> MPYEIFLAGVVSDNDEAKARAVLGGFTEMREHHRFTRVQHYEPQDIKIRGFPTIKELLKERGPTTALYQELHNILVRQPYTLQI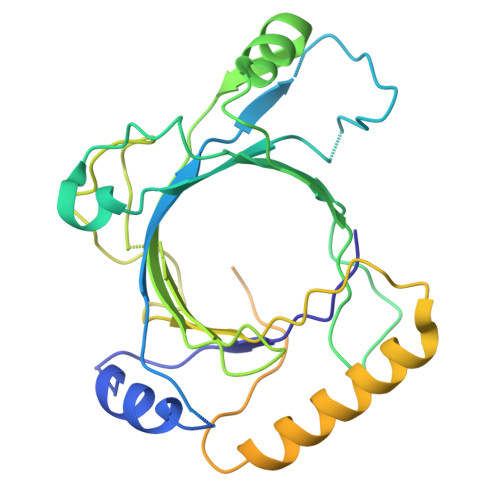RTNITDAILGPAQAGAEAAPHGTVSGGKPHILRWSDIPDPPNQRIPPFITQRKIIEIPDQRAPRILAASKFRNKSDLVEESYHWWFNDVEYSMVRTYLISLDPSPQTTDQVPSLAGLEPIGDFWLLYVRMRVEATPDRMQQAHNQLQQIRDQLLGVFEFKVWDRRAHDTRIMEQPTQGNGNVIGDAHNSNKKSNGVSPTTASSSEEVSPVDSQLTIPLPDDDDGDNVEDTPDTEMDEDDDESEYDSDSERDWPKDD>[2x]MDNPEAEPDDAVLFVGVSLVLGIASRHLLRGTRVPYTVALLVLGVALGSLEFGTKHGMGKLGAGIRIWANINPDLLLAVFLPALLFESSFSMEIHQIKKCMAQMVLLAGPGVLISTFFLGSALKLTFPYNWNWKTSLLLGGLLSATDPVAVVALLKELGASKKLSTIIEGESLMNDGTAIVVYQLFYRMVLGRTFDAGSIIKFLSEVSLGAVALGLAFGIASVLWLGFIFNDTIIEIALTLAVSYIAFFTAQDALEVSGVLTVMTLGMFYAAFAKTAFKGDSQQSLHHFWEMVAYIANTLIFILSGVVIADGVLENNVHFERHGASWGFLLLLYVFVQISRILVVVILYPLLRHFGYGLDLKEATILVWAGLRGAVALSLSLSVKRASDAVQTHLKPVDGTMFVFFTGGIVFLTLIFNGSTTQFLLHLLGMDRLAATKLRILNYTKYEMLNKALEAFGDLRDDEELGPPADWVTVKKYITCLNDLDDEPVHPHAVSDRNDRMHTMNLRDIRVRLLNGVQAAYWGMLEEGRITQTTANILMRSVDEAMDLVPTQELCDWKGLRSNVHFPNYYRFLQMSRLPRRLITYFTVERLESGCYICAAFLRAHRIARRQLHDFLGDSEVARIVIDESNAEGEEARKFLEDVRVTFPQVLRVLKTRQVTYSVLTHLSEYIQNLQKTGLLEEKEMAHLDDALQTDLKKFKRNPPLVKMPRVSDLLNTHPLVGALPAAMRDPLLSSTKETVKGHGTILYREGSRPTGIWLVSIGVVKWTSQRLSSRHSLDPILSHGSTLGLYEVLIGKPYICDMITDSVVHCFFIEAEKIEQLRQSDPSIEIFLWQESALVVARLLLPMMFEKMAT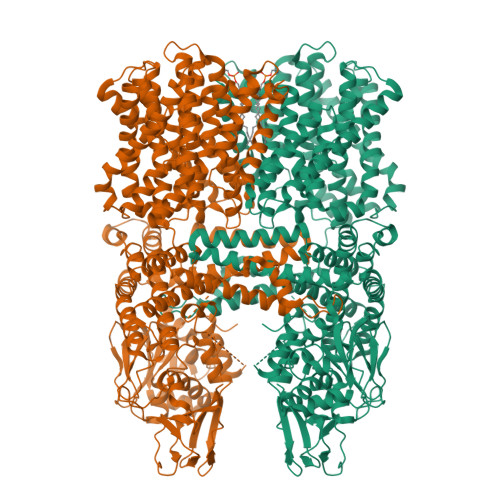HELRVLITERSTMNIYIKGEEIELEQNFIGILLEGFLKTKNQTLITPPGLLLPPNADLNLFGLESSAINRIDYCYTAPSYQVEARARILFVEIGRPEIEADLQRSASLISQTLELPRTQSKEHSGLLSWPESFRKSRGAQNGASLTEIRDHPASFSARALQLSMYGSMINDMKSGQGQGQRRQRHRHTKASSNKAHSSSYPRVPSRSSNTQRPLLSVQSEGANMTTARQAAAAGASLPPEPEEAGRRRRRQRKAIEEDEDNSSDESAGEEVIVRVDSPSMLTFRQPSSAADR>[3x]MGSSHHHHHHSQGSMTDDKDVLRDVWFGRIPTCFTLYQDEITEREAEPYYLLLPRVSYLTLVTDKVKKHFQKVMRQEDISEIWFEYEGTPLKWHYPIGL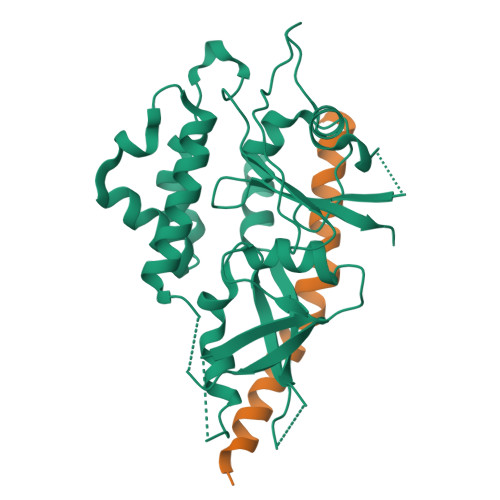LFDLLASSSALPWNITVHFKSFPEKDLLHCPSKDAIEAHFMSCMKEADALKHKSQVINEMQKKDHKQLWMGLQNDRFDQFWAINRKLMEYPAEENGFRYIPFRIYQTTTERPFIQKLFRPVAADGQLHTLGDLLKEVCPSAIDPEDGEKKNQVMIHGIEPMLETPLQWLSEHLSYPDNFLHISIIPQPTD;>MSSGLRAADFPRWKRHISEQLRRRDRLQRQAFEEIILQYNKLLEKSDLHSVLAQKLQAEKHDVPNRHEI[3x]>[2x]MHHHHHHEENVKRRTHNVLERQRRNELKR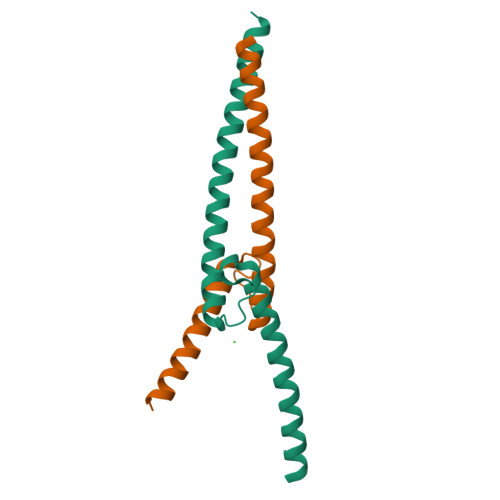SFFALRDQIPELENNEKAPKVVILKKATAYILSVQAEEQKLISEEDLLRKRREQLKHKLEQLRNS;>MADKRAHHNALERKRRDHIKDSFHSLRDSVPSLQGEKASRAQILDKATEYIQYMRRKNHTHQQDIDDLKRQNALLEQQVRALE[2x]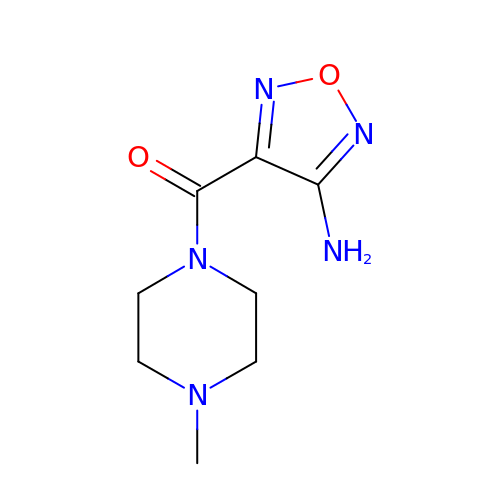(4-amino-1,2,5-oxadiazol-3-yl)(4-methylpiperazin-1-yl)methanone | C8 H13 N5 O2 | KQKPEPOSSQPUOT-UHFFFAOYSA-N>GQPPDHGDWTYEEQFKQLYELDGDPKRK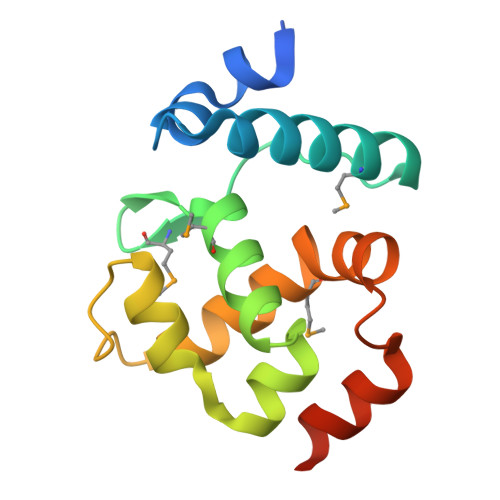EFLDDLFSFMQKRGTPVNRIPIMAKQVLDLFMLYVLVTEKGGLVEVINKKLWREITKGLNLPTSITSAAFTLRTQYMEYLYPYECEKRGLSNPNELQAAIDSNRREGRR[2x]4,5,6,7-TETRABROMO-BENZIMIDAZOLE 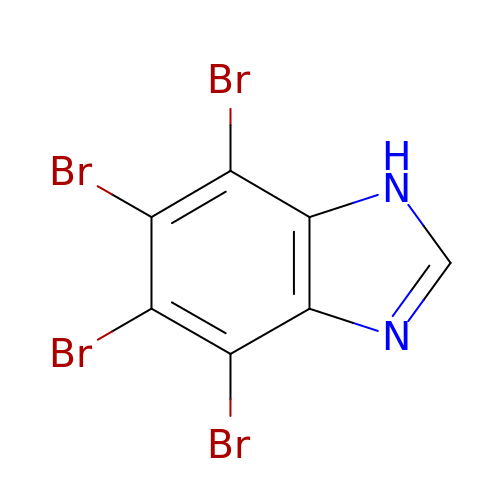| C7 H2 Br4 N2 | LOEIRDBRYBHAJB-UHFFFAOYSA-N> MSQEIRQNEKISYRIEGPFFIIHLMNPDNLNALEGEDYIYLGELLELADRNRDVYFTIIQSSGRFFSSGADFKGIAKAQGDDTNKYPSETSKWVSNFVARNVYVTDAFIKHSKVLICCLNGPAIGLSAALVALCDIVYSINDKVYLLYPFANLGLITEGGTTVSLPLKFGTNTTYECLMFNKPFKYDIMCENGFISKNFNMPSSNAEAFNAKVLEELREKVKGLYLPSCLGMKKLLKSNHIDAFNKANSVEVNESLKYWVDGEPLKRFRQLGSKQRKHR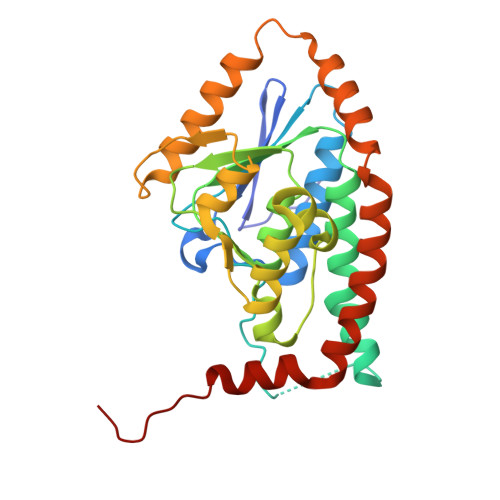L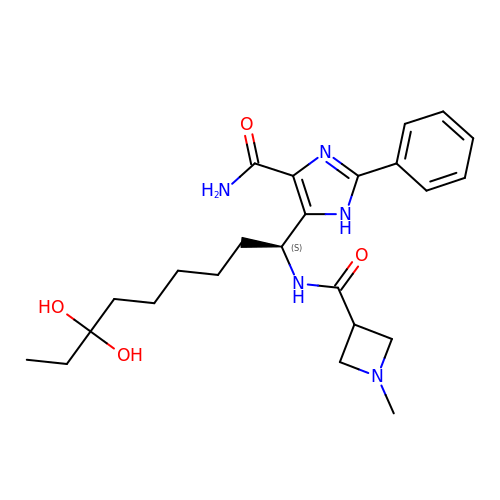5-{(1S)-7,7-dihydroxy-1-[(1-methylazetidine-3-carbonyl)amino]nonyl}-2-phenyl-1H-imidazole-4-carboxamide | C24 H35 N5 O4 | MYVMGGDKZVVQFO-SFHVURJKSA-N> MQHLDIAELVRSALEVSGCDPSLIGGIDSHSTIVLDLFALPSICISVKDDDVWIWAQLGADSMVVLQQRAYEILMTIMEGCHFARGGQLLLGEQNGELTLKALVH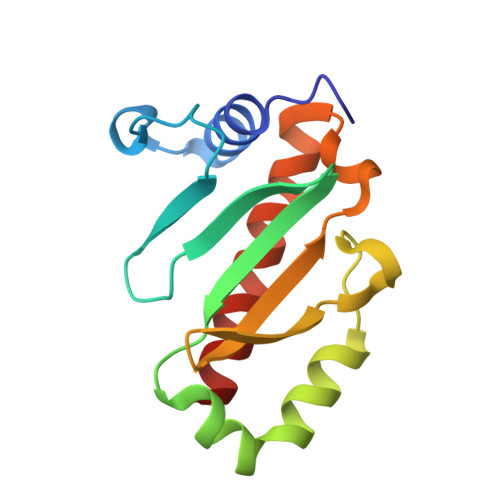PDFLSDGEKFSTALNGFYNYLEVFSRSLMR>MKMASSDASPSDGSTANLVPEVNNEVMALEPVVGAAIAAPVAGQQNVIDPWIRNNFVQ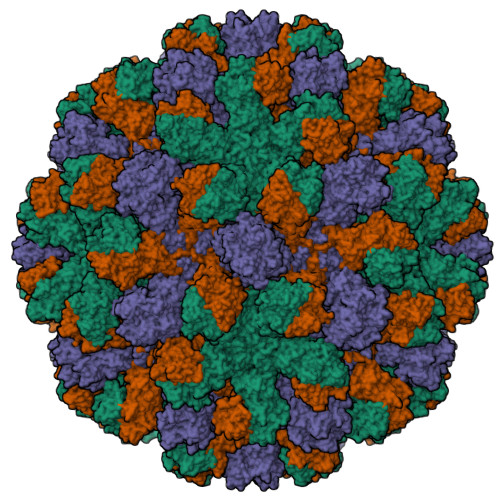APGGEFTVSPRNAPGEILWSAPLGPDLNPYLSHLARMYNGYAGGFEVQVILAGNAFTAGKIIFAAVPPNFPTEGLSPSQVTMFPHIIVDVRQLEPVLIPLPDVRNNFYHYNQSNDPTIKLIAMLYTPLRANNAGDDVFTVSCRVLTRPSPDFDFIFLVPPTVESRTKPFTVPILTVEEMTNSRFPIPLEKLFTGPSGAFVVQPQNGRCTTDGVLLGTTQLSPVNICTFRGDVTHIAGTHDYTMNLASQNWNNYDPTEEIPAPLGTPDFVGKIQGVLTQTTRGDGSTRGHKATVSTGSVHFTPKLGSVQFTTDTNNDLETGQNTKFTPVGVVQDGNSAHQNEPQQWVLPNYSGRTGHNVHLAPAVAPTFPGEQLLFFRSTMPGCSGYPNMNLDCLLPQEWVLHFYQEAAPAQSDVALLRFVNPDTGRVLFECKLHKSGYVTVAHTGPHDLVIPPNGYFRFDSWVNQFYTLAPMGNGAGRRRAL[3x]Here we report protein crystal structures of a piscine betanodavirus, the Grouper nervous necrosis virus (GNNV), in four different forms. The overall topological structure of the GNNV CP consists of the N-terminal arm (N-arm) (residues 34−51), the shell domain (S-domain) (residues 52−213), the linker region (residues 214−220) and the protrusion domain (P-domain) (residues 221−338). The S-domain comprises an eight-stranded anti-parallel β-sandwich with three short α-helices, which is a canonical structural feature similar to other virus CPs. The P-domain folds into an independent structure, including eight anti-parallel β-strands and a short α-helix connected with loops of various lengths.

To gain more complete and detailed structural information, we have determined the crystal structure of the truncated P-domain (residues 214−338) at high resolution (1.2 Å). Since it lacks only the S-domain, crystal packing of the truncated P-domain remains a trimer in the ASU, with a similar orientation and formation as the P-domains in the GNNV-LP. The high-resolution structure of the truncated P-domain has allowed us to clearly locate two Ca2+ ions near the non-crystallographic three-fold axis, which are coordinated with the C’-D’ loop to stabilize the trimeric structural fold. 275 motif on the C’-D’ loop from each neighboring subunit interacts with two Ca2+ ions and two water molecules through electrostatic and hydrogen-bonding interactions. This calcium-binding site is buried in the cavity of the protrusion at a distance of ~37 Å from the S-domain. Notably, only two of the three Asp275 residues are asymmetrically coordinated to the two Ca2+ ions, and the other Asp275 coordinates with one water molecule. There are two water molecules at the calcium-binding site providing the trimeric contacts and stabilizing the protrusion. At the interface between the D’ and E’ strands with the F’-G’ loop from neighboring subunits, we also find two invariant water molecules associated with 278VYWH281, Gly299, Gln322 and Ile323 through hydrogen bonds, which are also essential to maintain the conformation and stability of each of the trimeric P-domains. We consistently find three glycerol (GOL) molecules located between the B’-C’ and F’-G’ loops of the three P-domains, and one polyethylene glycol (PEG) molecule at the interface between the two F’-G’ loops from neighboring subunits. Notably, all these residue variations are located on the surface of the protrusion in the structure of the truncated P-domain. Our study identifies a PEG-binding site on the P-domain of GNNV CP and confirms the enhancement of GNNV infection in presence of PEG.

>NPEETTAPIMTQGSLYNDSLSTNDFKSILLGSTPLDIAPDGAVFQLDRPLSIDYSLGTGDVDRAVYWHLKKFAGNAGTPAGWFRWGIWDNFNKTFTDGVAYYSDEQPRQILLPVGTVCTRVDSEN[3x]>GGAAGUGUACCUAGGGAUCCACCUCGAGAGAGGAAGGACCAAGCGGUACAGGCCUACUUCGGUAGGUUACACCGUGGGGAUAAAAGA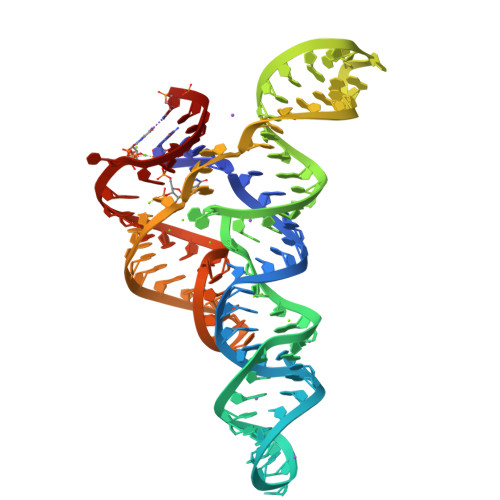CCCGUGGCAAGUUUC[2x]> HHHMLHLLEQIRAYCETCWEWQEAHEPGMDQDKNPMPAPVEHQICPAVCVLMKLSFDEEHRHAMNELGGLQAIAELLQVDCEMYGLTNDHYSITLRRYAGMALTNLTFGDVANKATLCSMKGCMRALVAQLKSESEDLQQVIASVLRNLSWRADVNSKKTLREVGSVKALMECALEVKKESTLKSVLSALWNLSAHCTENKADICAVDGALAFLVGTLTYRSQTNTLAIIESGGGILRNVSSLIATNEDHRQILRENNCLQTLLQHLKSHSLTIVSNACGTLWNLSARNPKDQEALWDMGAVSMLKNLIHSKHKMIA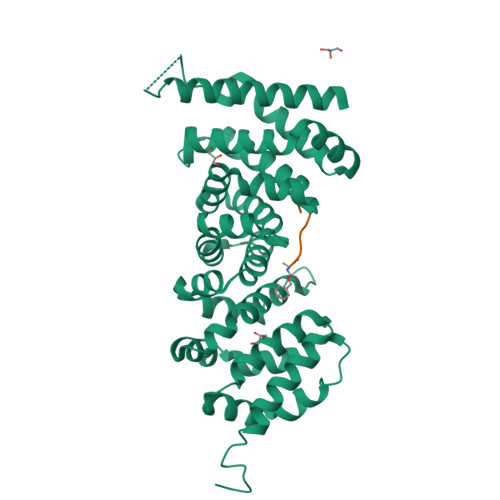MGSAAALRNLMANRPAKYKDAN>MGHHHHHHMKPYYVTTAIAYPNAAPHVGHAYEYIATDAIARFKRLDRYDVRFLTGTDEHGLKVAQAAAAAGVPTAALARRNSDVFQRMQEALNISFDRFIRTTDADHHEASKELWRRMSAAGDIYLDNYSGWYSVRDERFFVESETQLVDGTRLTVETGTPVTWTEEQTYFFRLSAYTDKLLAHYHANPDFIAPETRRNEVISFVSGGLDDLSISRTSFDWGVQVPEHPDHVMYVWVDALTNYLTGAGFPDTDSELFRRYWPADLHMIGKDIIRFHAVYWPAFLMSAGIELPRRIFAHGFLHNRGEKMSKSVGNIVDPVALAEALGVDQVRYFLLREVPFGQDGSYSDEAIVTRINTDLANELGNLAQRSLSMVAKNLDGRVPNPGEFADADAALLATADGLLERVRGHFDAQAMHLALEAIWLMLGDANKYFSVQQPWVLRKSESEADQARFRTTLYVTCEVVRIAALLIQPVMPESAGKILDLL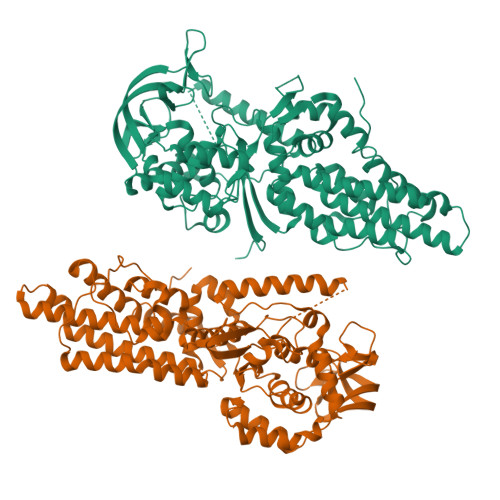GQAPNQRSFAAVGVRLTPGTALPPPTGVFPRYQPPQPPEGKRSHHHHHH[2x]>MNYARFITAASAARNPSPIRTMTDILSRGPKSMISLAGGLPNPNMFPFKTAVITVENGKTIQFGEEMMKRALQYSPSAGIPELLSWLKQLQIKLHNPPTIHYPPSQGQMDLCVTSGSQQGLCKVFEMIINPGDNVLLDEPAYSGTLQSLHPLGCNIINVASDESGIVPDSLRDILSRWKPEDAKNPQKNTPKFLYTVPNGNNPTGNSLTSERKKEIYELARKYDFLIIEDDPYYFLQFNSGRVPTFLSMDVDGRVIRADSFSKIISSGLRIGFLTGPKPLIERVILHIQVSTLHPSTFNQLMISQLLHEWGEEGFMAHVDRVIDFYSNQKDAILAAADKWLTGLAEWHVPAAGMFLWIKVKGINDVKELIEEKAVKMGVLMLPGNAFYVDSSAPSPYLRASFSSASPEQMDVAFQVLAQ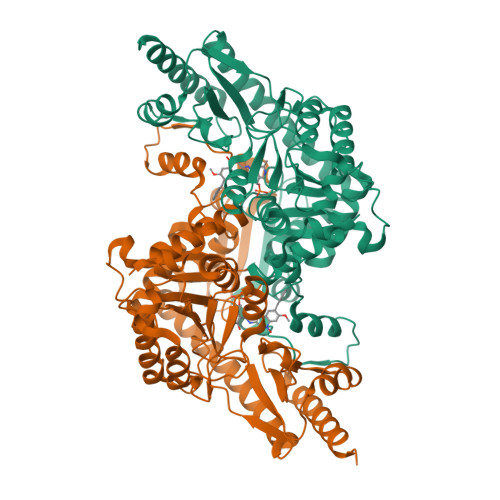LIKESLLVPRGSLEHHHHHH[4x]> MKNVGFIVTKSEIGGAQTWVNEISNLIKEECNIFLITSEEGWLTHKDVFAGVFVIPGIKKYFDFLTLFKLRKILKENNISTLIASSANAGVYARLVRLLVDF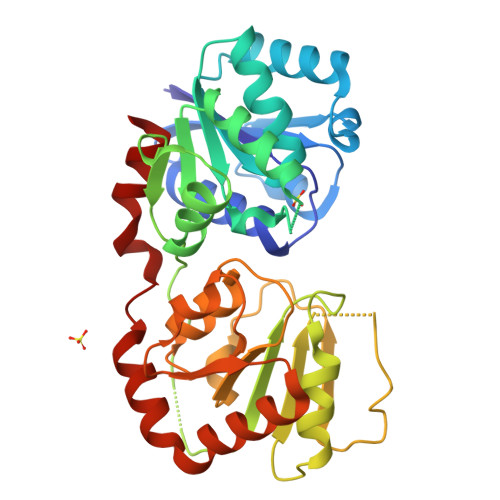KCIYVSHGWSCLYNGGRLKSIFCIVEKYLSLLTDVIWCVSKNDEKKAIENIGIKEPKIITVSNSVPQMPRCNNKQLQYKVLFVGRLTHPKRPELLANVISKKPQYSLHIVGGGERLESLKKQFSECENIHFLGEVNNFYNYHEYDLFSLISDSEGLPMSGLEAHTAAIPLLLSDVGGCFELIEGNGLLVENTEDDIGYKLDKIFDDYENYREQAIRASGKFVIENYASAYKSIILG The best characterized system is bacteriorhodopsin (bR), a light-driven proton pump, due to its biochemical robustness. The retinal chromophore of bR (Halobacterium salinarum) is linked to the side chain of Lys216 via a protonated Schiff base (PSB). Photon absorption by all-trans retinal triggers a functional photocycle consisting of a series of distinct spectroscopic intermediates (I→J→K→L→M→N→O) with sub-ps (I), ps (J), µs (K, L) and ms (M, N, O) lifetimes. Deprotonation of the Schiff base of photoisomerized 13-cis retinal and protonation of Asp85 during the L→M transition ultimately results in proton translocation to the extracellular side of the membrane.

The time delays between the optical laser flash (145 fs, 532 nm, 5.9 µJ, ~500 GW cm−2 in the interaction region, see “Methods” section) and the probing XFEL pulse were nominally 0.5, 1, 3 and 10 ps and 33 ms. Data from the nominally 0.5-ps delay were binned into 12 groups according to their actual time delay covering 0.24–0.74 ps. Within the first time point of 0.24 ps, the C9=C10 bond also distorts and undulates on the sub-ps timescale, while the C13=C14 bond torsion mostly progresses. The largest displacements, in opposite directions, are at atoms C14 and C10, while C8 undergoes minor distortion in the same direction as C10. The temporal evolution of the apparent C13=C14 dihedral angle can be separated in three distinct phases: 0–~500 fs (I), ~500–750 fs (II), 1–10 ps (III). In the present multiphoton regime, i.e. beyond the two-photon regime characterized by the spectroscopic data (≤180 GW cm−2), the situation most likely involves population of several all-trans excited states Sn followed by ultrafast multi-path electronic relaxation (≤0.5 ps, phase I) leading to hot populations in S0 and S1, with distorted retinal conformations and longer vibrational relaxation times on the electronic excited potential energy surface, compared to the single-photon regime. The C12-C13=C14-C15 torsion angle changes from −150° to −135° during 0.24–0.74 ps and refined to −112° at 1 ps and −100° at 3 ps. To accommodate the shifted Wat402, the carboxylate group of Asp85 reorients within 0.24 ps; the Asp212 χ2 torsion angle as well as distances between the carboxylate oxygen atoms of Asp212 and Wat402 show an oscillatory behaviour (~80 cm−1). Analysis of electron density maps calculated from extrapolated structure factors with varying occupancy of the pumped state yielded an occupancy of ~15% for the sub-ps and 1 ps data (10% for 3, 10 ps).

> QAQITGRPEWIWLALGTALMGLGTLYFLVKGMGVSDPDAKKFYAITTLVPAIAFTMYLSMLLGYGLTMVPFGGEQNPIYWARYADWLFTTPLLLLDLALLVDADQGTILALVGADGIMIGTGLVGALTKVYSYRFVWWAISTAAMLYILYVLFFGFTSKAESMRPEVASTFKVLRNVTVVLWSAYPVVWLIGSEGAGIVPLNIETLLFMVLDVSAKVGFGLILLRSRAIFGEAE> MLQPVFTLKLRHKISPRMVAVGRYDGTHPCLAAATQAGKVFIHNPHSRSQHLGAPRVLQSPLESDVSLLNINQTVSCLTAGVLNPELGYDALLVGTQTNLLAYDVYNNSDLFYREVADGASAIVLGTLGDITSPLAIIGGNCALQGFNHEGNDLFWTVTGDNVHSLALCDFDGDGKKELLVGSEDFDIRVFKEDEIVAEMSETEIITSLCPMYGSRFGYALSNGTVGVYDKTARYWRIKSKNQAMSIHAFDLNSDGVCELITGWSNGKVDARSDRTGEVIFKDNFSSAIAGVVEGDYRMEGCQQLICCSVDGEIRGYLPGTAEMRGNLMDISVEQDLIRELSQKKQNLLLELRNYEENAKAELSSPLNEADGHRGVIPANTKHHTALSVSLGSEAQAAHAELCISTSNDTIIRAVLIFAEGVFAGESHVVHPSVHHLSSSVRIPITPPKDIPVDLHLKTFVGYRSSTQFHVFELTRQLPRFSMYALTSPDPASEPLSYVNFIIAERAQRVVMWLNQNFLLPEDTNIQNAPFQVCFTSLRNGGQLYIKIKLSGEITVNTDDIDLAGDIIQSMASFFAIEDLQVEADFPVYFEELRKVLVKVDEYHSVHQKLSADMADNSNLIRSLLVQAEDARLMRDMKTMKNRYKELYDLNKDLLNGYKIRCNNHTELLGSLKAVNQAIQRAGHLRVGKPKNQVITACRDAIRSNNINMLFRIMRVGTASS;> MDLNLNRADYLQVGVTSQKTMKLLPASKHRATQKVVVGDHDGIVMCFGMKKGEAVTVFKTLPGQKIARLELGGALNTPQEKIFIAAGSEIRGFTKRGKQFLSFETNLTESIKAMHISGSDLFLSASYIYNHYCDCKDQHYYLSGDKINDVICLPVERLLREVPVLACQDRVLRVLQGSDVTYEIEVPGPPTVLALHNGNGGDSGEDLLFGTSDGKLGLIQITTSKPIHKWEIRNEKKRGGILCVDSFDIVGDGVKDLLVGRDDGMVEVYGFDNANEPVLRFDHTLSESVTSIQGGCVGKDGYDEIVVSTYSGWITGLTTEPVHKESGPGEELKFNQEMQNKISSLRSELEQLQYKVLQEREKYQQSSQSSKAKSAVPSFSVNDKFTLNKDDASYSLILEVQTAIDNVLIQSDVPIDLLDVDKNSAVVSFSSCDSESNDNFLLATYRCQANTTRLELKIRSIEGQYGTLQAYVTPRIQPKTCQVRQYHIKPLSLHQRTHFIDHDRPMNTLTLTGQFSFSELHSWVVFCMPEVPEKPPAGECVTFYFQNTFLDTQLESTYRKGEGVFKSDNISTISILKDVLSKEATKRKINLNISYEINEVSVKHTLKLIHPKLEYQLLLAKKVQLIDALKELQVHEGNTNFLIPEYRCILEEADHLQEEYKKQPAHLERLYGMITDLFIDKFKFKGTNVKTKVPLLLEILDSYDQNALIAFFDAA;> MAATSSSDSDGGKGESEANSKWLDSLSDSMANIHTFSACLALADFHGDGEYKLAMGDLGPDGRQPRLKVLKGHTLVSQKPLPDLPAAAVTFLMASHEPRTPALAIASGPCVYVYKNLKPYFKFSLPSLPTNPLEQDLWNQAKEDQIDPLTLKEMLEGIREKAEVPLSVQSLRFLPLELSEMEAFVNQHKSKSIRRQTVITTMTTLKKNLADEDAVSCLVLGTENKELLVLDPEAFTILAKMSLPSVPAFLEASGQFDVEFRLAAACRNGSIYILRRDSKRPKYCIELGAQPVGLVGVHKVLVVGSNQDSLHGFTYKGKRLWTVQMPAAILAMNLLEQHSRGLQAVMAALANEEVRIYHDKVLLNVIRTPEAVTSLCFGRYGREDNTLIMTTLGGGLIIKILKRTAVFAEGGGEAGPPPSQAIKLNVPRKTRLYVDQTLREREAGTAMHRTFQADLYLLRLRAARAYVQALESSLSPVSLTAREPLKLHAVVQGLGPTFKLTLHLQNTSTARPILGLVVCFLYNEVLYALPRAFFKVPLLVPGLNYPLETFVKSLSDKGISDIIKVLVLREGQSTPLLSAHINMPMSEGLAAD;> MAEEKLSARTQLPVSAESQKPVLKKAPEFPILEKQNWLIHLYYIQKDYEACKAVIKEQLQETHGLCEYAIYVQALIFRLEGNIQESLRLFQMCAFLSPQCADNLKQVARSLFLLGKHKAAIEVYNEAAKLNQKDWEICHNLGVCYIYLKQFDKAQDQLHNALHLNRHDLTYIMLGKIFLLKGDLDKAIEIYKKAVEFSPENTELLTTLGLLYLQLGIYQKAFEHLGNTLTYDPTNYKAILAAGSMMQTHGDFDVALTKYKVVACAVIESPPLWNNIGMCFFGKKKYVAAISCLKRANYLAPLDWKILYNLGLVHLTMQQYASAFHFLSAAINFQPKMGELYMLLAVALTNLEDSENAKRAYEEAVRLDKCNPLVNLNYAVLLYNQGEKRDALAQYQEMEKKVNLLKYSSSLEFDPEMVEVAQKLGAALQVGEALVWTKPVKDPKSKHQTASTSKAAGFQQPLGSNQALGQAMSSAATCRKLSSGAGGTSQLTKPPSLPLEPEPTVEAQPTEASAQTREK;> MEPLLLAWSYFRRRRFQLCADLCTQMLEKSPCDQAAWILKARALTEMVYVDEIDVDEEGIAEMILDENAIAQVPRPGTSLKLPGTNQTGGPSPAVRPVTQAGRPITGFLRPSTQSGRPGTIEQAIKTPRTAYTARPIASSSGRFVRLGTASMLTSPDGPFINLSRLNLAKYAQKPKLAKALFEYIFHHENDVKTALDLAALSTEHSQYKDWWWKVQIGKCYYRLGLYREAEKQFKSALKQQEMVDTFLYLAKVYISLDQPLTALNLFKQGLDKFPGEVTLLCGIARIYEEMNNISSATEYYKEVLKQDNTHVEAIACIGSNHFYTDQPEVALRFYRRLLQMGVYNCQLFNNLGLCCFYAQQYDMTLTSFERALSLAENEEEVADVWYNLGHVAVGTGDTNLAHQCFRLALVSNNQHAEAYNNLAVLEMRRGHVEQAKALLQTASSLAPHMYEPHFNFATISDKIGDLQRSYAAAKKSEAAFPDHVDTQHLIKQLEQHFAML;> MSVLDALWEDRDVRFDVSSQQMKTRPGEVLIDCLDSVEDTKGNNGDRGRLLVTNLRIVWHSLALPRVNLSIGYNCILNITTRTANSKLRGQTEALYVLTKCNSTRFEFIFTNLVPGSPRLYTSLIAVHRAYETSKMYRDFKLRSALIQNKQLRLLPQENVYNKINGVWNLSSDQGNLGTFFITNVRIVWHANMNDSFNVSIPYLQIRSVKIRDSKFGLALVIESSQQSGGYVLGFKIDPVEKLQESVKEINSLHKVYSANPIFGVDYEMEEKPQPLEALTVKQIQDDVEIDSDDHTDAFVAYFADGNKQQDREPVFSEELGLAIEKLKDGFTLQGLWEVMN;> MAETKSMFREVLPKQGQLYVED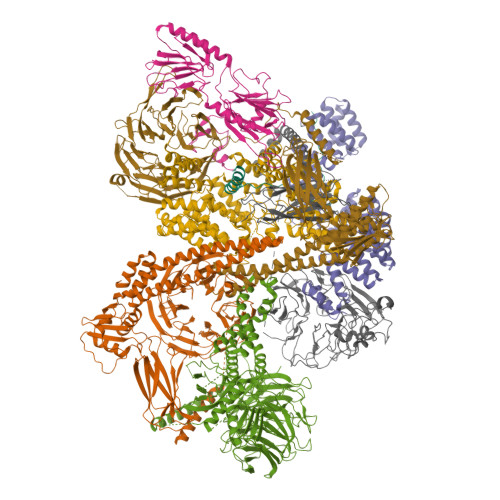ITTMVLCKPKLLPLKSLTLEKLEKMQQAAQDTIHQQEMTEKEQKITH;> MSLFKARDWWSTVLGDKEEFDQGCLCLADVDNTGNGQDKIIVGSFMGYLRIFNPHPVKTGDGAQAEDLLLEVHLRDPILQVEVGKFVSGTEMLHLAVLHSRKLCVYSVSGTLGNVEHGNQYQIKLMYEHNLQRTACNMTYGSFGGVKGRDLICIQSVDGMLMVFEQESYAFGRFLPGSLLPGPLAYSSRTDSFITVSSCHQVESYKYQVLAFATDADKRQETEQQKHGSGKRLVVDWTLNIGEQAIDICIVSFIQSASSVFVLGERNFFCLKDNGQIQFMKKLDYSPSCFLPYCSVSEGTINTLIGNHNNMLHIYQDVTLKWATQLPHVPVAVRVGCLHDLKGVIVTLSDDGHLQCSYLGTDPSLFQAPKVESRELNYDELDMELKELQKVIKNVNKSQDVWPLTEREDDLKVSAMVSPNFDSVSQATDVEVGADLVPSVTVKVTLKNRVALQKIKLSIYVQPPLVLTGDQFTFEFMAPEMTRTVGFSVYLKGSYSPPELEGNAVVSYSRPTERNPDGIPRVSQCKFRLPLKLVCLPGQPSKTASHKLTIDTNKSPVSLLSLFPGFAKQSEDDQVNVMGFRFLGGSQVTLLASKTSQRYRIQSEQFEDLWLITNELIIRLQEYFEKQGIKDFTCSFSGSVPLEEYFELIDHHFELRINGEKLEELLSERAVQFRAIQRRLLTRFKDKTPAPLQHLDTLLDGTYKQVIALADAVEENQDNLFQSFTRLKSATHLVILLIGLWQKLSADQIAILEAAFLPLQQDTQELGWEETVDAALSHLLKTCLSKSSKEQALNLNSQLGIPKDTSQLKKHITLFCDRLAKGGRLCLSTDAAAPQTMVMPGGCATIPESDLEGRSIDQDSSELFTNHKHLMVETPVPEVSPLQGVTE CueO plays an important role in copper homeostasis by oxidation of toxic cuprous ions to cupric ions. As with all multi-copper oxidases, it contains four copper atoms distributed within one type 1 (T1)2 copper site and a trinuclear cluster comprising the T2 and T3 copper sites. A distinguishing feature of CueO is a partially structured 45-amino acid segment (residues 356–404) capping the entrance to the T1/sCu copper-binding sites. The goal of the current study was to engineer the highly compliant MRS such that CueO activity would be modulated by engagement of a partner protein with a scaffolded peptide.

To gain further mechanistic insights, we determined crystal structures of both the free and MDM2(6–125)-bound forms of CueO-PM2 along with CueO-12.1. The asymmetric unit for the MDM2-bound form comprised a single binary complex with the scaffolded PM2 peptide adopting its prototypical α-helical conformation. The three key signature residues (Phe, Trp, and Leu) projecting from the outer face of the helix are accommodated by discrete pockets in a prolonged hydrophobic cleft of MDM2. Comparison with structures of unscaffolded PMI, a related stapled derivate (MO6, differing by one amino acid), and the parental p53 peptide bound to MDM2 (32, 36, 41) shows highly similar side chain conformations of these residues. The adjacent MRS residues Met-396 and Asn-397 extend the PM2 α-helix to more fully occupy the MDM2 binding groove. The PM2 conformation is further stabilized by hydrophobic interactions between residues on its inner face (Leu-393 and Tyr-390) and Ile-358 and Met-361 on the α5 helix. In addition to a polar contact between side chains of Lys-94 of MDM2 and Gln-365 in the α5 helix, these interactions likely drive ordering of the MRS linker residues abutting PM2 that are highly mobile in native CueO. The MDM2-bound PM2 helix is positioned well away from the sCu and T1 copper-binding sites, permitting unhindered access to Cu and syringaldazine substrates and resulting in the observed MDM2-dependent activity gains. The structure of MDM2 bound to CueO-PM2 showed clear dislocation of the PM2 insert away from the sCu and T1 copper-binding sites, rescuing enzymatic activity. In the case of CueO-PM2, co-incubation with MDM2 resulted in ∼1.6-fold increased kcat (and no change in Km).

> AERPTLPIPDLLTTDARNRIQLTIGAGQSTFGGKTATTWGYNGNLLGPAVKLQRGKAVTVDIYNQLTEETTLHWHGLEVPGEVDGGPQGIIPPGGKRSVTLNVDQPAATCWFHPHQHGKTGRQVAMGLAGLVVIEDDEILKLMLPKQWGIDDVPVIVQDKKFSADGQIDYQLDVMTAAVGWFGDTLLTNGAIYPQHAAPRGWLRLRLLNGCNARSLNFATSDNRPLYVIASDGGLLPEPVKVSELPVLMGERFEVLVEVNDNKPFDLVTLPVSQMGMAIAPFDKPHPVMRIQPIAISASGALPDTLSSLPALPSLEGLTVRKLQLSMDPILDMMGMQMLMEKYGDQAMAGMDHSQMTSFAEYWALLSMNHGGKFDFHHANKINGQAFDMNKPMFAAAKGQYERWVISGVGDMMLHPFHIHGTQFRILSENGKPPAAHRAGWKDTVKVEGNVSEVLVKFNHDAPKEHAYMAHCHLLEHEDTGMMLGFTVKDPNSSSVDKLAAALEHHHHH;> GPMSVPTDGAVTTSQIPASEQETLVRPKPLLLKLLKSVGAQKDTYTMKEVLFYLGQYIMTKRLYDEKQQHIVYCSNDLLGDLFGVPSFSVKEHRKIYTMIYRNLVVVNQQESSDSGTSVSEN> IGTGFPFDPHYVEVLGERMHYVDVGPRDGTPVLFLHGNPTSSYLWRNIIPHVAPSHRCIAPDLIGMGKSDKPDLDYFFDDHVRYLDAFIEALGLEEVVLVIHDWGSALGFHWAKRNPERVKGIACMEFIRPFPTWDEWPEFARETFQAFRTADVGRELIIDQNAFIEGALPKYVVRPLTEVEMDHYREPFLKPVDR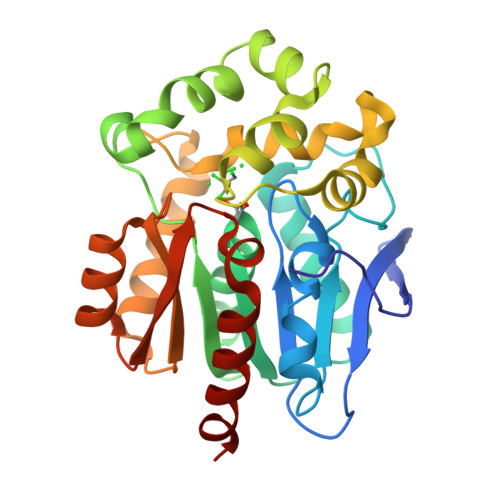EPLWRFPNELPIAGEPANIVALVEAYMNWLHQSPVPKLLFWGTPGFIIPPAEAARLAESLPNCKTVDIGPGLHFLQEDNPDLIGSEIARWLPALHH The COP1 E3 ubiquitin ligase is a central signaling hub that integrates inputs from plant light‐sensing photoreceptors. COP1 contains an N‐terminal zinc finger, a central coiled‐coil, and a C‐terminal WD40 domain, which is essential for proper COP1 function (Deng et al, 1992; McNellis et al, 1994). COP1 regulates gene expression and plays a central role as a repressor of photomorphogenesis by directly modulating the stability of transcription factors that control the expression of light‐regulated genes.

We tested this by mutating residues Lys422, Tyr441, and Trp467 in the VP peptide binding pocket of COP1. The COP1Lys422Ala mutant binds HY539–48 as wild type, but increases the binding affinity of UVR8406–413 ~ 10‐fold. A UVR8406–413–COP1Lys422Ala complex structure reveals the UVR8 VP peptide in a different conformation, with UVR8Tyr407 binding at the surface of the VP‐binding pocket. Interestingly, COP1Lys422Ala interacts with full‐length UVR8 also in the absence of UV‐B in yeast two‐hybrid assays, which is not detectable for wild type COP1 (Rizzini et al, 2011). Moreover, COP1Lys422Ala also interacts more strongly with the constitutively interacting UVR8C44 fragment (corresponding to the C‐terminal UVR8 tail containing the VP motif) when compared to wild type COP1 in yeast two‐hybrid assays. The COP1Lys422Ala mutant binds UV‐B‐activated full‐length UVR8 with wild type affinity, while COP1Trp467Ala binds ~ 5 times more weakly. The COP1Lys422Ala mutation can modulate the interaction with different VP peptide. Unexpectedly, COP1Lys422Ala rendered the UVR8 protein unstable, preventing conclusive analysis of the effect of this COP1 mutant on UV‐B signaling in vivo.

> GAMTFTRYSRLRVIAEIRHGDIFHSANIVSSIEFSDRDDELFATAGVSRCIKVFDFSSVVNEPADMQCPIVEMSTRSKLSCLSWNKHEKNHIASSDYEGIVTVWDVTTRQSLMEYEEHEKRAWSVDFSRTEPSMLVSGSDDCKVKVWCTRQEASVINIDMKANICCVKYNPGSSNYIAVGSADHHIHYYDLRNISQPLHVFSGHKKAVSYVKFLSNNELASASTDSTLRLWDVKDNLPVRTFRGHTNEKNFVGLTVNSEYLACGSETNEVYVYHKEITRPVTSHRFGSPDMDDAEEEAGSYFISAVCWKSDSPTMLTANSQGTIKVLVLAA;> XRYAVVPDE> GMALEPQIKSAPTPVILIVEPYGGSIRQQNPNLPMVFWDDAALTRGDGIFETLLIRDGHACNVRRHGERFKASAALLGLPEPILEDWEKATQMGIESWYSHPNAGEASCTWTLSRGRSSTGLASGWLTITPVSSDKLAQREHGVSVMTSSRGYSID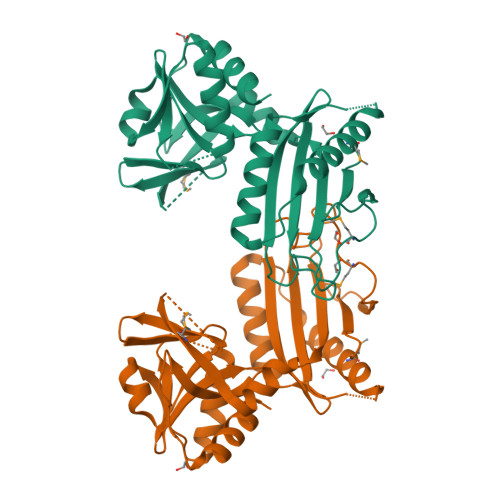TGLPGIGKATRGELSKVERTPAPWLTVGAKTLAYAANMAALRYAKSNGFDDVIFTDGDRVLEGATSTVVSFKGDKIRTPSPGGDILPGTTQAALFAHATEKGWRCKEKDLSIDDLFGADSVWLVSSVRGPVRVTRLDGHKLRKPDNEKEIKALITKALG> SESDSEMVPFPQLPMPIENNYRACTIPYRFPSDDPKKATPNEISWINVFANSIPSFKKRAESDITVPDAPARAEKFAERYAGILEDLKKDPESHGGPPDGILLCRLREQVLRELGFRDIFKKVKDEENAKAISLFPQVVSLSDAIEDDGKRLENLVRGIFAGNIFDLGSAQLA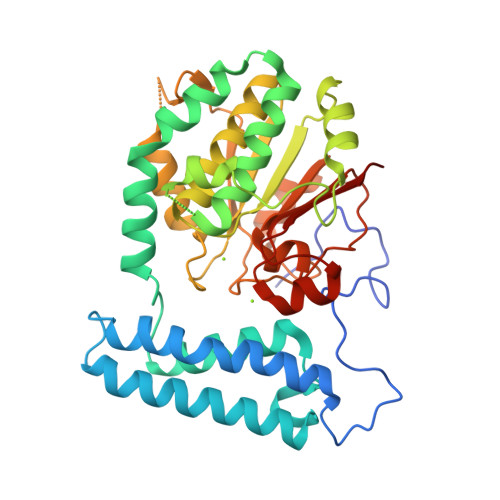EVFSRDGMSFLASCQNLVPRPWVIDDLENFQAKWINKSWKKAVIFVDNSGADIILGILPFARELLRRGAQVVLAANELPSINDITCTELTEILSQLKDENGQLLGVDTSKLLIANSGNDLPVIDLSRVSQELAYLSSDADLVIVEGMGRGIETNLYAQFKCDSLKIGMVKHLEVAEFLGGRLYDCVFKFNEVQS MONOVACCENIN | C21 H40 O4 | 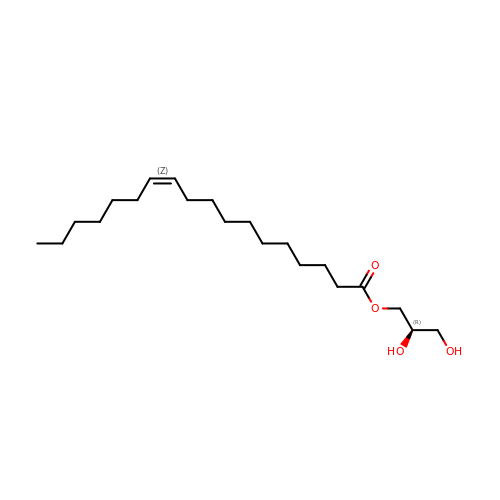KJHYUSLWTPMFTN-WHXUGTBJSA-N>TRAASASPAPGTGATPDGFSAEESLEEIDGAVSPGPSDAPDGEYGDLDARTAVRAAATERDRFYVCPPPSGSTVVRLEPEQACPEYSGGSGNDMLSRIAAAWCELQ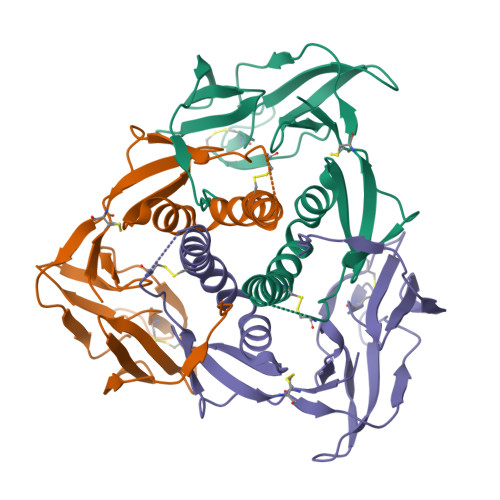NKDRTLWGEMSRLNPSAVATAALGQRVSARMLGDVMAISRCVEVRGGVYVQNSMRVPGERGTCYSRPLVTFEHNGTGVIEGQLGDDNELLISRDLIEPCTGNHRRYFKLGGGYVYYEDYSYVRMVEVPETISTRVTLNLTHHHHHHHH[6x]>MNTNKATATYLKSIMLPETGPASIPDDITERHILKQETSSYNLEVSESGSGVLVCFPGAPGSRIGAHYRWNANQTGLEFDQWLETSQDLKKAFNYGRLISRKYDIQSSTLPAGLYALNGTLNAATFEGSLSEVESLTYNSLMSLTTNPQDKVNNQLVTKGVTVLNLPTGFDKPYVRLEDETPQGLQSMNGAKMRCTAAIAPRRYEIDLPSQRLPPVPATGTLTTLYEGNADIVNSTTVTGDINFSLAEQPADETKFDFQLDFMGLDNDVPVVTVVSSVLATNDNYRGVSAKMTQSIPTENI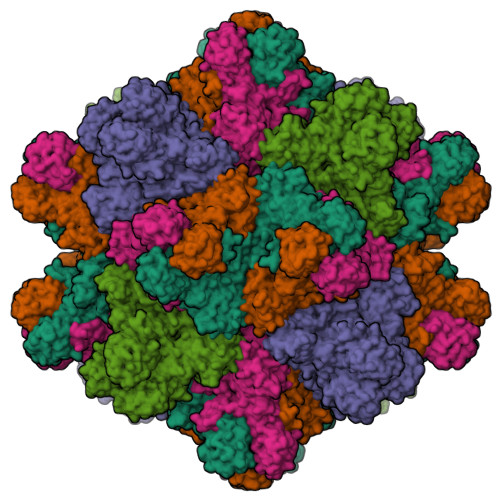TKPITRVKLSYKINQQTAIGNVATLGTMGPASVSFSSGNGNVPGVLRPITLVAYEKMTPLSILTVAGVSNYELIPNPELLKNMVTRYGKYDPEGLNYAKMILSHREELDIRTVWRTEEYKERTRVFNEITDFSSDLPTSKA[5x]> MSAVKKQRIDLRLTDDDKSMIE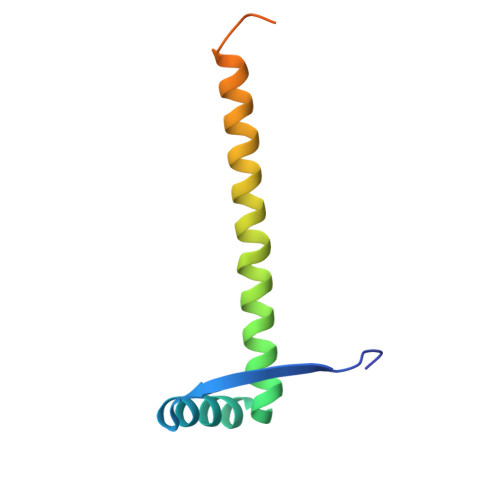EAAAISNQSVSQFMLNSASQRAAEVIEQHRRVILNEESWTRVMDALSNPPSPGEKLKRAAKRLQGM>MRFETLQLHAGYEPEPTTLSRQVPIYPTTSYVFKSPEHAANLFALKEFGNIYSRIMNPTVDVLEKRLAALEGGKAALATASGHAAQFLALTTLAQAGDNIVSTPNLYGGTFNQFKVTLKRLGIEVRFTSREERPEEFLALTDEKTRAWWVESIGNPALNIPDLEALAQAAREKGVALIVDNTFGMGGYLLRPLAWGAALVTHSLTKWVGGHGAVIAGAIVDGGNFPWEGGRYPLLTEPQPGYHGLRLTEAFGELAFIVKARVDGLRDQGQALGPFEAWVVLLGMETLSLRAERHVENTLHLAHWLLEQPQVAWVNYPGLPHHPHHDRAQKYFKGKPGAVLTFGLKGGYEAAKRFISRLKLISHLANVGDTRTLAIHPASTTHSQLSPEEQAQAGVSPEMVRLSVGLEHVEDLKAELKEALA[2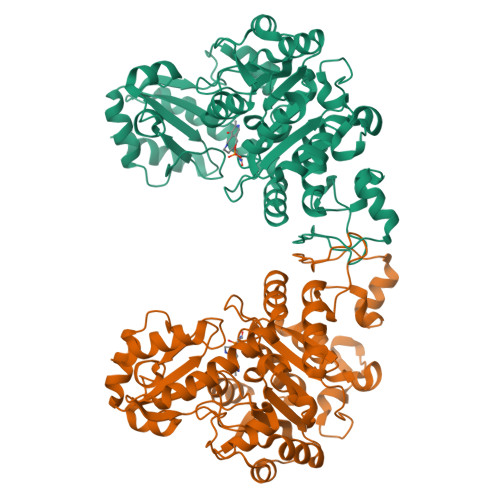x]> SLM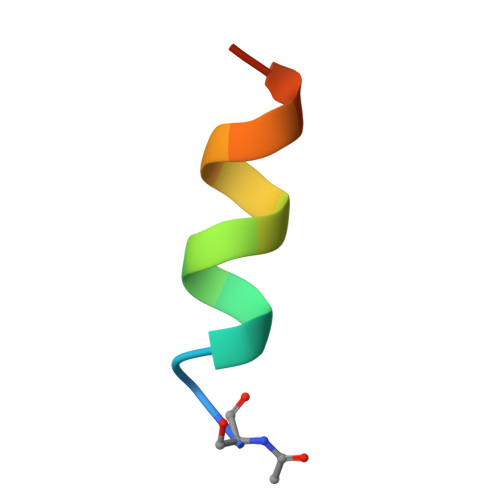RVQAHIRKRMVA> SQANLMRLKSDLFNRSPMYPGPTKDDPLTVTLGFTLQDIVKVDSSTNEVDLVYYEQQRWKLNSLMWDPNEYGNITDFRTSAADI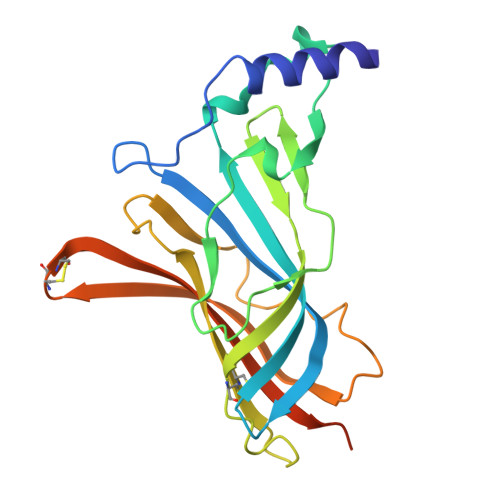WTPDITAYSSTRPVQVLSPQIAVVTHDGSVMFIPAQRLSFMCDPTGVDSEEGVTCAVKFGSWVYSGFEIDLKTDTDQVDLSSYYASSKYEILSATQTRQVQHYSCCPEPYIDVNLVVKFRERRAGNGFFRNLFDHHHHHH(5-HYDROXY-4-{[(3-HYDROXYISOXAZOL-4-YL)AMINO]METHYL}-6-METHYLPYRIDIN-3-YL)METHYL 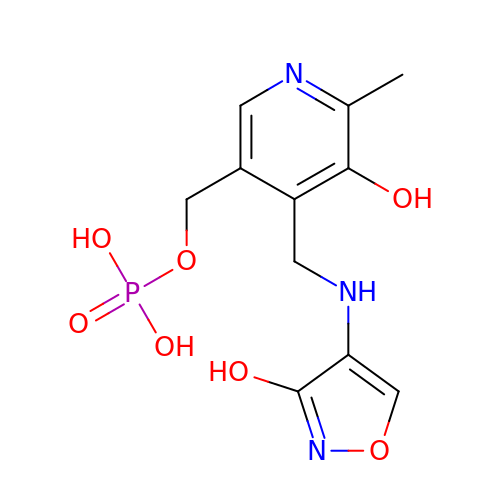DIHYDROGEN PHOSPHATE | C11 H14 N3 O7 P | PXWFNGNWQUPGPJ-UHFFFAOYSA-N>[2x]LAFNEPLNVVSHLNHDWFLFGDSRSDCNHINNLKIKNFDYLDIHPSLCNNGKISSSAGDSIFKSFHFTRFYNYTGEGDQIIFYEGVNFNPYHRFKCFPNGSNDVWLLNKVRFYRALYSNMAFFRYLTFVDIPYNVSLSKFNSCKSDILSLNNPIFINYSKEVYFTLLGCSLYLVP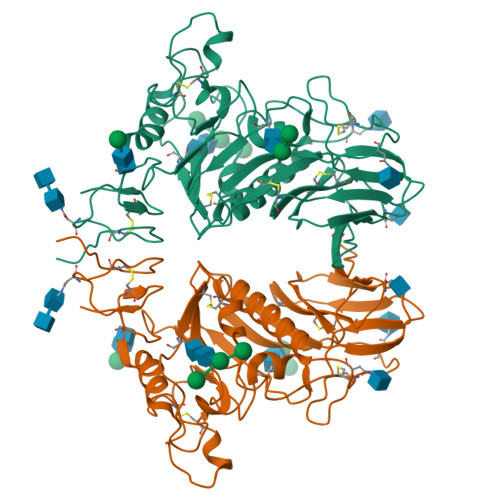LCLFKSNFSQYYYNIDTGSVYGFSNVVYPDLDCIYISLKPGSYKVSTTAPFLSLPTKALCFDKSKQFVPVQVVDSRWNNERASDISLSVACQLPYCYFRNSSANYVGKYDINHGDSGFISILSGLLYNVSCISYYGVFLYDNFTSIWPYYSFGRCPTSSIIKHPICVYDSDPLVPR> 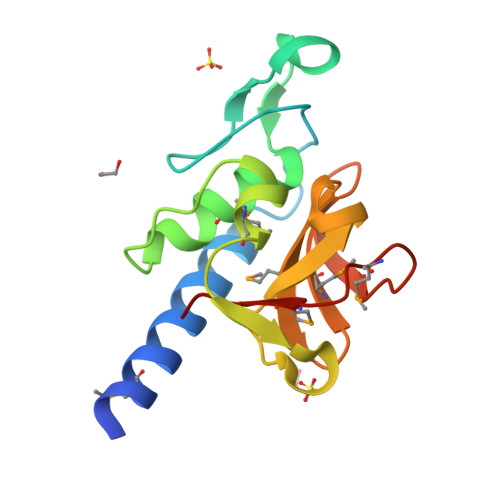ATADPGVRAMDYQQATDVVIARGLSQRGVPFSWAGGGINGPTRGTGTGANTVGFDASGLMQYAYAGAGIKLPRSSGAMYRVGQKILPQQARKGDLIFYGPEGTQSVAMYLGNNQMLEVGDVVQVSPVRTAGMAPYMVRVLGT> MGSSHHHHHHSQDPMDLERYAIVVSAAVEADELVLDLDKSTLEELEAKLNQELAGTDQVGEQAGKELAEGLERGAVEGLDVRQVLAKLKAALKGEVRELATEEVKALRAAIQHALGVELDDNAKRQLAESAKLLDRIIESATRNQSLTVKLRFDADRSALLTAERLADAYLNRIREALKQDKSSPLYQAFSALAKGTGEKLSPDEAKFRAGLFADVRDRFLALLKQDLQSYIADQLKRGHAVGDIKLPDTQAILSEAGLPTLKQALLLSRAVDLDANNRAKLAKDLGQFMPEVAQVLKAPEKGASWEEINAVVREAKKAIHDAEEARRVALSLRSVTKEGNKPFAQQTGRFHTIELQEEGSPDEFQELLRLQASTQGHVDETTLARLVVQKRATKAILKKLLETADRPEEQAVWRAAIERLVIGNTAYDLKDDESFAKLIELAKKHPLEKVVKNVREVQFSEKVTLSDKYAFVPASNQGRIFLSHLRRENIYRTPTQRPLSLKVAEEGEGVRLKEMEEKALGDGALGILRPQSLGLPEDYTGVVQVRGELADPEGNVYAGLKGTVIVDPRAKEDFLNLNDLYRGDTVVDGKKYTKEEVDALIREKLKTGALQLNLGIHRVSTVEEAKVGKQVFLRHMGGVPFNRGRISPSEAAKWAAQAKELKFLPMIAGREMGLSHYQQIATLAKTFGVEVDEGQYSMAASHTAYKELDPEIYRLLEEGVELDAEGRPIVPIVIGKEMAAKLGLKEGDIAFTFRNPVMGHGGALLQARVAAIRDRLNAVVVNQEYAKSTGVDFDGDTLVVLPKGLPVDPHRLEVFQTLMAHAGLAGGRKGGGSVEPSPGELRFKEQLEVYDKVLARLSKSRLAAELRNAGVEDLSNPFEVVRQLESLGEEELLKAFKGYLRKGFAKELGLDLKSEEDRARLNQYLFEGFLDYRKQFQDPRRVYKKLPLMPSAALAASLLQVEAHKKEYDPSDPVALAAGQLTTSFLGLSEKLAQDLETSIDFPKLAEAIRAYNQAYSSGNEEQVAKARAELVKVLNDPTVQKFSLSNLLYQIITDRKKRDYSLRVRTESGKTYEYRNLYAVLNRLMQNLPVEEVADTVYDASGQAVEERVPLKQSATRSLVKGLLDLASGKVKEDPDGTVAEDLADLPVFGELEQLYGLVADAKYDPSSLKSALVKPNKPQGSYAEITTLLYRGIANQEGLAETNLPRDEVAR

Many bacterial and eukaryotic viruses with double-stranded DNA genomes in the realms Duplodnaviria and Varidnaviria encode homologs of cellular RNAPs (collectively denoted “two-barrel RNAPs”). The TMP-fused virion RNAP transcribes pre-early phage genes, including a gene that encodes another, non-virion RNAP, that transcribes early and some middle phage genes. Transcription by vRNAP and nvRNAP is directed by dissimilar AT-rich and GC-rich promoters, respectively, and the two phage RNAPs have distinct overall architectures, with the TMP-fused vRNAP being unusually flat and lacking the clamp domain.

Thus, the N-terminal part of the giant gp96 TMP protein appears to be a virion RNAP (vRNAP) that could be responsible for the transcription of the phage early genes. Several N-terminal fragments of gp96 containing the RNAP signature motif were cloned, purified, and tested for the ability to extend the RNA component of an RNA-DNA scaffold that mimics the conformation of nucleic acids within the transcription elongation complex of other RNAPs. While the shortest gp96 1050-residue fragment was inactive, 1200-, 1360- and 1540-residue fragments extended the primer. We crystallized the 1–1200 and 327–1124 fragments and determined their structures at 3.1 Å and 4.4 Å resolution, respectively. The structure of the 1–1200 fragment was largely the same as the structure of the 327–1124 fragment because most of the flanking regions not essential for the activity were disordered, except for two helices at the C-terminus (1125–1162). The overall architectures of gp96 vRNAP and gp64 nvRNAP are markedly different. In contrast, gp96 vRNAP contains no defined domain at the corresponding position, resulting in a clamp-less, flat structure that heretofore has not been observed for any RNAP. We hypothesize that this unique structure enables the passage of gp96 vRNAP through the narrow channel in the phage tail. Gp96 is exceptional as it lacks the C-terminal region, and its connector element, which is disordered in the gp96 crystals (gp96 613–679), is twice shorter than in QDE-1 and phi14:2. The disordered region is likely positioned close to the RNA-DNA hybrid duplex during transcription elongation and might dynamically interact with the nascent RNA strand, moving similarly to the clamp domains of other RNAPs.> PASLTEIEHLVQSVCKSYRETCQLRLEDLLRQRSNIFSREEVTGYQR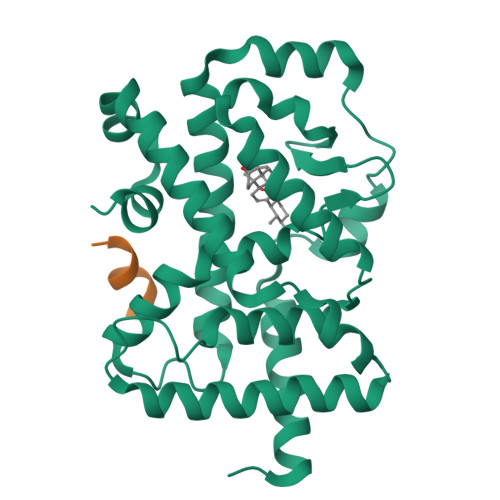KSMWEMWERCAHHLTEAIQYVVEFAKRLSGFMELCQNDQIVLLKAGAMEVVLVRMCRAYNADNRTVFFEGKYGGMELFRALGCSELISSIFDFSHSLSALHFSEDEIALYTALVLINAHRPGLQEKRKVEQLQYNLELAFHHHLCKTHRQSILAKLPPKGKLRSLCSQHVERLQIFQHLHPIVVQAAFPPLYKELFSTE;> KILHRLLQ> MAAPGAGPGPGAPPGLEAALQKLALRRKKVLSAEETELFELAQAAGGAMDPEVFKILVDLLKLNVAPLAVFQMLKSMCAG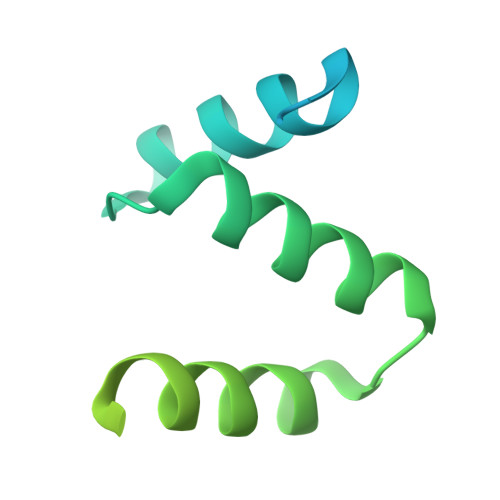QRLASEPQDPVAVPLPTTSVPETRGRNRGSSALGGGPALAERSGREGSSQRMPRQPSATRLPKGGGPGKSPTRST The ncAA l-enduracididine is an early intermediate in guanitoxin biosynthesis and is produced by GntC, a unique pyridoxal-5′-phosphate (PLP)-dependent enzyme. GntC catalyzes a cyclodehydration from a stereoselectively γ-hydroxylated l-arginine precursor via a reaction that functionally and mechanistically diverges from previously established actinobacterial cyclic arginine ncAA pathways. GntC initially facilitates the reversible deprotonations of the α- and β-positions of its substrate before catalyzing an irreversible diastereoselective dehydration and subsequent intramolecular cyclization. Consistent with many type I/II PLP-dependent enzymes, the GntC active site is found at the homodimer interface.

GntC crystallized as a dimer of homodimers and adopted a largely α-helical structural fold. PLP was bound to K219 in each monomer as an internal aldimine; this was consistent with sequence alignment results that suggested this lysine was responsible for anchoring the cofactor in the active site. PLP-bound and PLP-1 GntC structures were highly similar (0.31 Å root-mean-square deviation (RMSD) for backbone atom overlap) with the major structural difference being an additional N-terminal ordered helix that helps form the active site in the PLP-1-bound complex. When comparing PLP-bound and PLP-1 internal and external aldimine substrates, there was a 30° downward rotation of the pyridine ring, orienting the amino acid substrate toward a new ordered N-terminal helix that was not present in the first structure. The comparison of holo- and substrate-bound GntC structures and activity assays on site-specific mutants further identified amino acid residues that contribute to the overall catalytic mechanism.

>[4x]MKIQPALLEMWLSEYERVPYNLGESSVDNFTLGELLNLTGDRDALDQLSLMNNDTHGSLRLREAIASLDKSVSPDDILVTAGTTEAILIYFKVRYRSGANVVVPVPTFHVLYETPAFLGYEVRYLQLRAENGFRIDPQELAKLVDDNTEVIVLNTPQNPSGVVCSETEIQSIIEIAEKHNAEILADEHYRFLPHDQDTEILPSLYGLSPKIISLGSTGKCFGCIGLRIGWLIGNPEIIKACHFFKDYTTHTVCVLNDYIAAGVLLHKGKILPRYRQMIQHNIQQFETFIKQQRGLIDWVKPEAGTIAFPFFTDPNINSKIVAKRLVEDHGVLLLPGEAFDRPSHFRIALGVEPSLFQYALEKLAIVIETS>[2x]GPLGSMVSGVGGSGGGRGGGRGGEEEPSSSHTPNNRRGGEQAQSSGTKSLRPRSNTESMSKAIQQYTVDARLHAVFEQSGESGKSFDYSQSLKTTTYGSSVPEQQITAYLSRIQRGGYIQPFGCMIAVDESSFRIIGYSENAREMLGIMPQSVPTLEKPEILAMGTDVRSLFTSSSSILLERAFVAREITLLNPVWIHSKNTGKPFYAILHRIDVGVVIDLEPARTEDPALSIAGAVQSQKLAVRAISQLQALPGGDIKLLCDTVVESVRDLTGYDRVMVYKFHEDEHGEVVAESKRDDLEPYIGLHYPATDIPQASRFLFKQNRVRMIVDCNATPVLVVQDDRLTQSMCLVGSTLRAPHGCHSQYMANMGSIASLAMAVIINGNEDDGSNVASGRSSMRLWGLVVCHHTSSRCIPFPLRYACEFLMQAFGLQLNMELQLALQMSEKRVLRTQTLLCDMLLRDSPAGIVTQSPSIMDLVKCDGAAFLYHGKYYPLGVAPSEVQIKDVVEWLLANHADSTGLSTDSLGDAGYPGAAALGDAVCGMAVAYITKRDFLFWFRSHTAKEIKWGGAKHHPEDKDDGQRMHPRSSFQAFLEVVKSRSQPWETAEMDAIHSLQLILRDSFKESEAAMNSKVVDGVVQPCRDM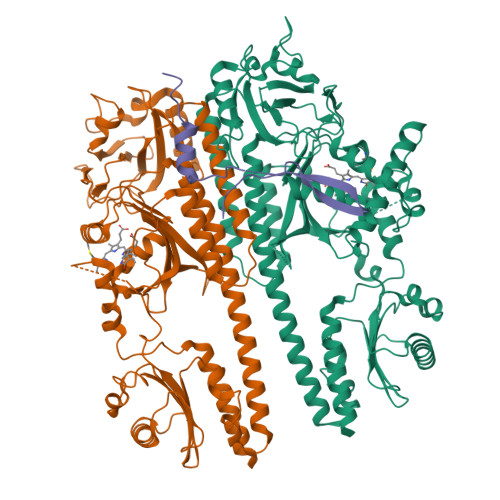AGEQGIDELGAVAREMVRLIETATVPIFAVDAGGCINGWNAKIAELTGLSVEEAMGKSLVSDLIYKENEATVNKLLSRALRGDEEKNVEVKLKTFSPELQGKAVFVVVNACSSKDYLNNIVGVCFVGQDVTSQKIVMDKFINIQGDYKAIVHSPNPLIPPIFAADENTCCLEWNMAMEKLTGWSRSEVIGKMIVGEVFGSCCMLKGPDALTKFMIVLHNAIGGQDTDKFPFPFFDRNGKFVQALLTANKRVSLEGKVIGAFCFLQIPSPELQQALAVQRRQDTECFTKAKELAYICQVIKNPLSGMRFANSLLEATDLNEDQKQLLETSVSCEKQISRIVGDMDLESIEDGSFVLKREEFFLGSVINAIVSQAMFLLRDRGLQLIRDIPEEIKSIEVFGDQIRIQQLLAEFLLSIIRYAPSQEWVEIHLSQLSKQMADGFAAIRTEFRMACPGEGLPPELVRDMFHSSRWTSPEGLGLSVCRKILKLMNGEVQYIRESERSYFLIILELPVPRKRPLSTASGSGDMMLMMPY;> GPLGSMMFLPTDYCCRLSDQEYMELVFENGQILAKGQRSNVSLHNQRTKSIMDLYEAEYNEDFMKSIIHGGGGAITNLGDTQVVPQSHVAAAHETNMLESNKHVD> ATMITSNQLGTITEDSGSYTPGTIATATRLVLTPRETPQSITVVTRQNMDDFGLNNIDDVMRHTPGITVSAYDTDRNNYYARGFSINNFQYDGIPSTARNVGYSAGNTLSDMAIYDRVEVLKGATGLLTGAGSLGATINLIRKKPTHEFKGHVELGAGSWDNYRSELDVSGPLTESGNVRGRAVAAYQDKHSFMDHYERKTSVYYGILEFDLNPDTMLTVGADYQDNDPKGSGWSGSFPLFDSQGNRNDVSRSFNNGAKWSSWEQYTRTVFANLEHNFANGWVGKVQLDHKINGYHAPLGAIMGDWPAPDNSAKIVAQKYTGETKSNSLDIYLTGPFQFLGREHELVVGTSASFSHWEGKSYWNLRNYDNTTDDFINWDGDIGKPDWGTPSQYIDDKTRQLGSYMTARFNVTDDLNLFLGGRVVDYRVTGLNPTIRESGRFIPYVGAVYDLNDTYSVYASYTDIFMPQDSWYRDSSNKLLEPDEGQNYEIGIKGEYL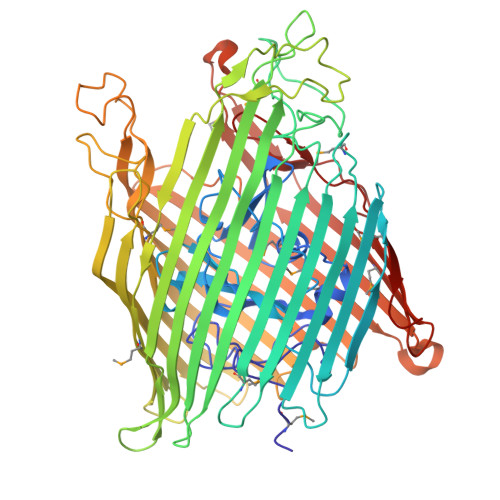DGRLNTSLAYFEIHEENRAEEDALYNSKPTNPAITYAYKGIKAKTKGYEAEISGELAPGWQVQAGYTHKIIRDDSGKKVSTWEPQDQLSLYTSYKFKGALDKLTVGGGARWQGKSWQMVYNNPRSRWEKFSQEDYWLVDLMARYQITDKLSASVNVNNVFDKTYYTNIGFYTSASYGDPRNLMFSTRWDF> HHHHHHNGNGEKIELTFMFRGQPQEQTAYKNVVKKFEEKHPNVKVNIVVTSPDQYATKLRAAIAGRKIPDVFYFNPGELRAYVNSNVLLDITKYVENSKGVNLQDIWEKGVNKYRFDGEKVGQGNLYGLPKDLGPFALG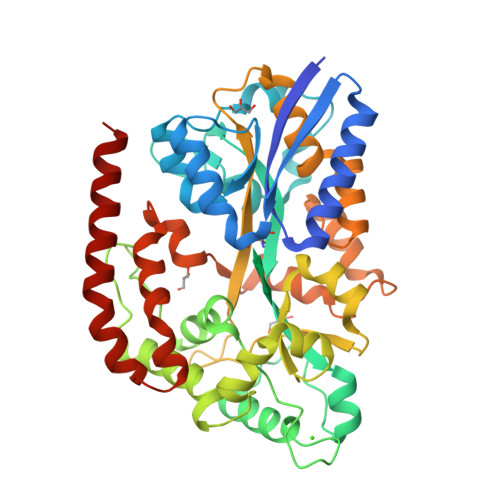YNKTMFEKAGIPLPDKDKPYTWQEFIDVCKKLTKDTNGDGKLDQWGTGLNATWTLQGFVWSNGADWIDESKTKVTVDDPKFIEALQFFADMQNKYKVTPSIAEAQTLDTYQRWLRGQLGFFPVGPWDLAAFDQQIKFEYDLIPWPAGSTGKPATWVGSLGIGVSSMTKHPKEAVELALYLSADPEGQKALVDQRVQLPNSVKVAEEWAKDPSIKPANKQEFLDIINDYGHSFPTEYTYNGEWYDEFYRNLQPVLDGKMSAEEYVKKAKPKMQKLLDQAIEQEKQASKK>GPLGSAYQLLLSKETLNKILQYKQNLEKGLATPGKFFLEELSKQEKSISEMDITTFTQLLIQSKKPQVFAESQVYHDGTDWTLEEESILGDVSVNMPVTMYNDGGHGSSFKNHPKPISGYLAYVPGALLASGSGPTSDMKEVLDNGKLNQDKLNALYERRLLPQLIHFNELARQNEKQAAITIPGIGTGCFSGAYYDVIKPYVRNALIHILEKHKDSLPYIDIIHYDPYMGDEPAEKKIGHMSFRVSPSGVVRGTTGQLDYPLGSNPDTHILVSIVAWDHFSWPGNDYWGGARQTDDGVKAASTDTMGQVTGATGVYDKKWGRYMPPESFTKDRKGMSDWGDYVRENGIVFNGPVLALDKSGKLDTLENVASRSSKAKVETTTTISDLVRSMFSLFSHS[8x]

ADP-ribosylation is a reversible post-translational modification involved in various cellular activities. Removal of ADP-ribosylation requires (ADP-ribosyl)hydrolases, with macrodomain enzymes being a major family in this category. Further analyses reveal DUF4804 as a class of MavL-like macrodomain enzymes whose representative members show unique selectivity for mono-ADP-ribosylated arginine residue in synthetic substrates. Crystal structures of several proteins in this class provide insights into arginine specificity and a shared mode of ADP-ribose interaction distinct from previously characterized macrodomains.

Here, we show that the Legionella macrodomain effector MavL regulates this pathway by reversing the arginine ADP-ribosylation, likely to minimize potential detrimental effects caused by the modified ubiquitin. As full-length recombinant MavL behaved poorly in expression and purification, we chose to proceed with MavL42-435, a construct that was recently crystallized and its structure reported. Our apo-MavL crystals belong to space group P1 21 1, with eight MavL molecules in the asymmetric unit. We then tried to capture MavL in its ADPR-bound form through co-crystallization of MavL with ADPR and soaking MavL-UbVME crystals with ADPR. Interestingly, the same R370-involving protomer:protomer interaction was observed in MavL crystals obtained from co-crystallization trials that failed to yield bound ADPR. Thus, it appears that the arginine insertion contributes to packing interactions outcompeting ADPR binding.>[2x]IKESVYVKSSLFSVFIFLSFYLGCLLVGFVHYLRFQRKSIDGSFGSNDGSGNMVASHPIAASTPEPDIESDKNIIRTKMFLYLSDLSRKDRRIVSK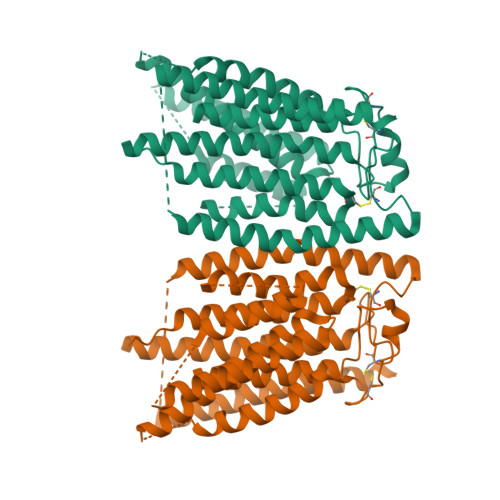KYKIYFWNIITIAVFYALPVIQLVITYQTVVNVTGNQDICYYNFLCAHPLGVLSAFNNILSNLGHVLLGFLFLLIVLRRDILHRRALEAKDIFAVEYGIPKHFGLFYAMGIALMMEGVLSACYHVCPNYSNFQFDTSFMYMIAGLCMLKLYQTRHPDINASAYSAYASFAVVIMVTVLGVVFGKNDVWFWVIFSAIHVLASLALSTQIYYMGRFKIDLGIFRRAAMVFYTDCIQQCSRPLYMDRMVLLVVGNLVNWSFALFGLIYRPRDFASYMLGIFICNLLLYLAFYIIMKLRSSEKVLPVPLFCIVATAVMWAAALYFFFQNLSSWEGTPAESREKNRECILLDFFDDHDIWHFLSATALFFSFLVLLTLDDDLDVVRRDQIPVFDYKDHDGDYKDHDIDYKDDDDK>[4x]GSGGRATMEPSALRKAGSEQEEGFEGLPRRVTDLGMVSNLRRSNSSLFKSWRLQCPFGNNDKQESLSSWIPENIKKKECVYFVESSKLSDAGKVVCQCGYTHEQHLEEATKPHTFQGTQWDPKKHVQEMPTDAFGDIVFTGLSQKVKKYVRVSQDTPSSVIYHLMTQHWGLDVPNLLISVTGGAKNFNMKPRLKSIFRRGLVKVAQTTGAWIITGGSHTGVMKQVGEAVRDFSLSSSYKEGELITIGVATWGTVHRREGLIHPTGSFPAEYILDEDGQGNLTCLDSNHSHFILVDDGTHGQYGVEIPLRTRLEKFISEQTKERGGVAIKIPIVCVVLEGGPGTLHTIDNATTNGTPCVVVEGSGRVADVIAQVANLPVSDIT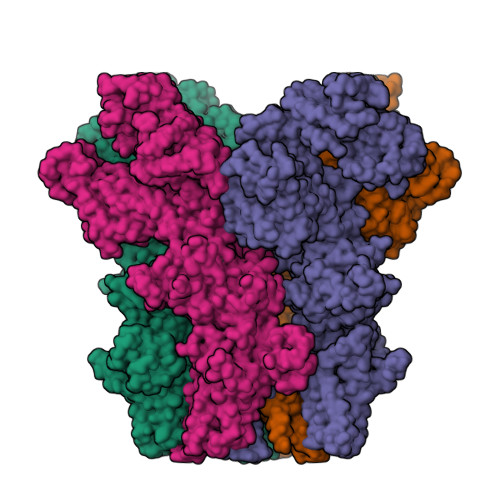ISLIQQKLSVFFQEMFETFTESRIVEWTKKIQDIVRRRQLLTVFREGKDGQQDVDVAILQALLKASRSQDHFGHENWDHQLKLAVAWNRVDIARSEIFMDEWQWKPSDLHPTMTAALISNKPEFVKLFLENGVQLKEFVTWDTLLYLYENLDPSCLFHSKLQKVLVEDPERPACAPAAPRLQMHHVAQVLRELLGDFTQPLYPRPRHNDRLRLLLPVPHVKLNVQGVSLRSLYKRSSGHVTFTMDPIRDLLIWAIVQNRRELAGIIWAQSQDCIAAALACSKILKELSKEEEDTDSSEEMLALAEEYEHRAIGVFTECYRKDEERAQKLLTRVSEAWGKTTCLQLALEAKDMKFVSHGGIQAFLTKVWWGQLSVDNGLWRVTLCMLAFPLLLTGLISFREKRLQDVGTPAARARAFFTAPVVVFHLNILSYFAFLCLFAYVLMVDFQPVPSWCECAIYLWLFSLVCEEMRQLFYDPDECGLMKKAALYFSDFWNKLDVGAILLFVAGLTCRLIPATLYPGRVILSLDFILFCLRLMHIFTISKTLGPKIIIVKRMMKDVFFFLFLLAVWVVSFGVAKQAILIHNERRVDWLFRGAVYHSYLTIFGQIPGYIDGVNFNPEHCSPNGTDPYKPKCPESDATQQRPAFPEWLTVLLLCLYLLFTNILLLNLLIAMFNYTFQQVQEHTDQIWKFQRHDLIEEYHGRPAAPPPFILLSHLQLFIKRVVLKTPAKRHKQLKNKLEKNEEAALLSWEIYLKENYLQNRQFQQKQRPEQKIEDISNKVDAMVDLLDLDPLKRSGSMEQRLASLEEQVAQTAQALHWIVRTLRASGFSSEADVPTLASQKAAEEPDAEPGGRKKTEEPGDSYHVNARHLLYPNCPVTRFPVPNEKVPWETEFLIYDPPFYTAERKDAAAMDPMGDTLEPLSTIQYNVVDGLRDRRSFHGPYTVQAGLPLNPMGRTGLRGRGSLSCFGPNHTLYPMVTRWRRNEDGAICRKSIKKMLEVLVVKLPLSEHWALPGGSREPGEMLPRKLKRILRQEHWPSFENLLKCGMEVYKGYMDDPRNTDNAWIETVAVSVHFQDQNDVELNRLNSNLHACDSGASIRWQVVDRRIPLYANHKTLLQKAAAEFGAHYFE> SEDEEDILARVDLETTRAIAKQMFSSGTVVEVSSDEEGFQGCWFAAKVVEPVGEDKFLVEYRDLREKDGIEPLKEETDFLHIRPPPPRDEDIDFAVGDKINAFYNDGWWVGVVIDGMKHGTVGIYFRQSQEKMRFGRQGLRLHKDWVDGTWQLPLKGGKIKRE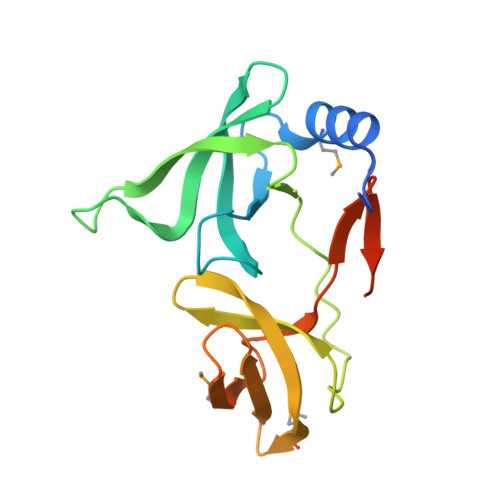KTVS>[2x]MRRHGFSLLELLLASVLMGSLLLVVLALENSSATLRERERARGRLADELSLTATVLARELYTVGYRLTGQALVLSPS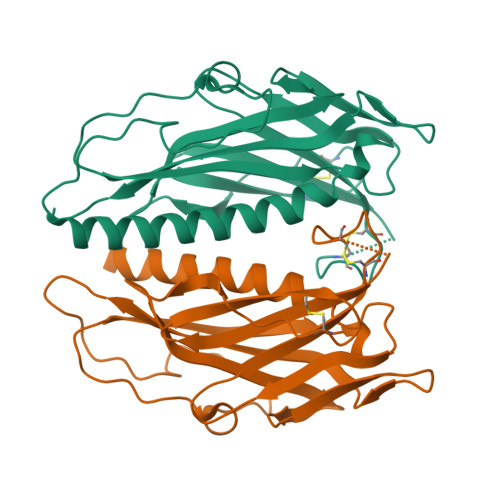SQGDGVQGWFLCEAGMEEICGESMGEVRGTGYEVNQGALRWGACKGEGCAPLPNNPVLGGDEVQVEAFRVAYLEGGTWKRQAQAVNLRPEGASPKVSALALYLLASVPVRGGAPAFTPGSTLSYPPGLTSSLLELPGAPNDGRLRAEKLWIVQTPNLAR>MISMKPRYKPDWESLREHTVPKWFDKAKFGIFIHWGIYSVPGWATPTGELGKVPMDAWFFQNPYAEWYENSLRIKESPTWEYHVKTYGENFEYEKFADLFTAEKWDPQEWADLFKKAGAKYVIPTTKHHDGFCLWGTKYTDFNSVKRGPKRDLVGDLAKAVREAGLRFGVYYSGGLDWRFTTEPIRYPEDLSYIRPNTYEYADYAYKQVMELVDLYLPDVLWNDMGWPEKGKEDLKYLFAYYYNKHPEGSVNDRWGV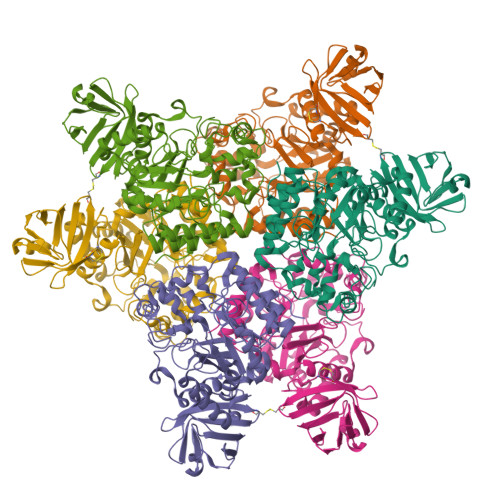PHWDFKTAEYHVNYPGDLPGYKWEFTRGIGLSFGYNRNEGPEHMLSVEQLVYTLVDVVSKGGNLLLNVGPKGDGTIPDLQKERLLGLGEWLRKYGDAIYGTSVWERCCAKTEDGTEIRFTRKCNRIFVIFLGIPTGEKIVIEDLNLSAGTVRHFLTGERLSFKNVGKNLEITVPKKLLETDSITLVLEAVEEHHHHHH[2x]> MFLIHFVHYKTILQKYTFKFKHIFLSIDKYNSLFFNISGILIWLNIIHINIILIKYSFFILINNFEYLIILIST;> MFRLTAASQKNLNSWYTKGTMRGGVPRIYYAWMRPGSFTRRRFEKMRNPFVDLETGTSLYFRDTRDSAEAIAHAADSKGIKGMDNAIDLYNEYRIVPDLYPEGFQWKHKLNTEYNQWRSNTWLTPDLIPKEHRGRFLCNFQLNIVAYDMRVVKFSPKDHRQWIYCVLYVGSGKGIAGWGRAVAPSTQEAKKEAIREAFSNIIAVDLEQEGPMYPVRVNADGVRVLLYPARRIVANFRVADILCAFGFQHAGCRINLKATNNPKSPTHTVEGVFEAVKALRSVSEIAASRGKVPHSLIYNIYPYLEEIRRRKGMMAMHPPGKDGLLMPDRVVDNRLPDHLKRGYYDDVYWKDFFAGSDEHLNEPRMGLRGDEMRRRLEEAQTSPAPTTAKDTRRRTLEDVLKRLGKTTRDLGSIPIVNPRVDVGLPTHIKRNYQLH;> MQKLLSPRTARHARLFRLAGKLADSGSPGVPKSDGERLVWVNSHVRRDKDISLSQEEERIRELMMPLEVGENSFAANGQATHGNLFYFREYPMYPGEYVPAEHNTLSSLRDELRLDLTAQSLKEAWMRVSGGVYFQSVDEYYASVDGLDAEQIGEVLAALFPELNCYEAQALVQRTLECISRPVSAASRQLSRTITAEAVGLDNAPGHYTNFLEWMGRLTETRAFKTEHALFEFSRRKFNRDDVRVMFENYRLMSKATLLADSADSYSHFYTVLKDFARKVAGEDSRHQIGVRIDEAEVDPETGIAVGRGCADGEKYHFTALLRENRDHNGIITVMGKPLSLVLDNKAWLMEMVLMPFDEANLDYRDFDAHIVSEGHAMPSIANEIAAFALRMAVANALVKLIPLTRIPLKKSGLLSVDRRRERGQFPGYLDGKKVKRRFAKR;> MVRRSHVVAYYWSRYRMPTQMPKFDGPAPVAAPQSMNSTKTNEFIDPIDDKFPMSIRGPLVRPDVPEDQYVDSWYICTSMTHHMGDYRPWSASAPPNAFRFRPFNEFDAKGREYVQYMREFARFDPRKSRGNGQKGFPFRDAYLTKMNEANQKTPPPTLETIMDRAVREHHQHARILSPLEVQRDVGRLEPIPSYAGKINADRSVFPFQWKTEDWYEYEVAKVRNRRFVFENTEEDGIRGSEVTYKIVLEGFWDHHVMKLAEDVCMFLKDVGRQIVEEKLVAVRRLLQGGAVDPELLAAFNCARAGPFGGLDEYDKEEVANFLRSDLRRLEEQCLSVINRCNVPVPGATNIYDPHTSWPHVEKLEPWVRMAEFWTSSSDTSFTELEMSTAHYEFRKFFRVIICKLPFQSTEFEKRMYDIRHWLHRQTSCEFHTIYRRNVIHDSAVFPTEHDPATPTTHEHHRMFSFALDWQSAPVNRLSTDTVHEGESWDAVAQRLGCSVGELKDANAERETIEAGVVINVPVTATRRLTSFGATPLVLPLKTTSAKDGERIRTWEEAAAILDCTVEELQQCNGHAALTYQKKESEAGEFDSSVTELVAPLSCWTSTSESEFSPVERVHANDTLVAIARRLQCSEEALRAVNDGITDVSGLDFVRVPPEARRPRRLVEPQLRPQAATDALLARTIAEEETFKLKSIPHLPQNAERFPHEYHTPTSRFPPTPSETPATQDWMAYTAKYLDKQFTISAEPAPVYNVNKLWPMQQIPGKVDQTPFEEDQTWLLHSIPVQQLEMHHHEKDLQDLPFINHEQFPRSLEWNAP;> MMRKSVTFLRRGKPRPRAGMFPDKYRRVPMLLKPQQGGQQYFNHFLIRSTNDRLTQQDVDNASGQAHSFISPQLPQMDWRNMSARSSEESIREEMRQLAENDVMQHQRVFNERMWYEKEEEHRMKARSCPEETSEHAISNDGAVPPPRVLGGDYFKTRFGYSLVKNSEMTQGPVDYSQLDMWGEMPRYTSDMVFLYLVSRRRNTYAVAYTYEGKRILNTYTAGNRGLKGGDRGFRSEGSTDNGHQVTSMYLNDLLPKLREMRASEGRPMGRGEKVELVVRVMGFYNGRQGAVRAVQDRANEFHVRYFEDITPFPLNGPKMPRGVFK;> MFCFSRGLWMRHIGQDVPKRHTHFVLESRLMYEKSFRDCWLHSVCRAISQLDEPLSKTVVGTHQKMLQRKVTCFQYNQYGLFKTPYYRLANVDRYHAVQGVAGTREWVPYVNVSYWTMNKMVRGGNLLVHRVHYTGWGTDSHLKKGGWEHRWNKVLQRNVLQYSRI;> MAFRNTFTTPGKFSTVSKNIVLLLIWRVKVFLRAEGFAHSLVMLPVSLYSKILLCDVKKKIVYFHCCTRKKSMLRRCPCVWPDGPTKSSVSIGTAFTLQKRFLKIAKSAFGFYLARRGQRKYPFLRRPHIKNTHSMNPSAPYFWSFMTAKSQMAFLPEENYITGDWTGKFFVSKRQVYTLQHATSGAKVRVKSFPSIFEFNSPSRWNIGKEMNTLTKPRMDLIDEQMLTKKQRLDYVRAGLLPK;> MRSKTLKKSLAAMYMRPPVTCYTDACEAPVAMWDGAIPLKETRKLKNGVPVRTVSRTYSHPPQLTPTQLSFNDINSMYCVGNDELIQFFPEGLGGRVFQTMPPGHPRGFLYRKETHLLNLFVDKVQHWHTKRSVLSSLTNGRTGFIVDGPTGCGKSALMCQVVHFARSRNIVTLYVPDAKVWTHGEWCWPSTILPGFFDAPDAARSFLKYFAVANRATLTSWKLRCTPKDLPTEQGERQPQNLYELCEWGHRAVAPASIDRQSVCVKFLMDELSEEKKLPVVIVVDGWNLFSHETHFRYPHPDFLRGLASFNESSTDIDLYPQELPRIPASRLSFVRGLNKMILSGDDPNKFFITCTTRDFKPFDGISGFPNVETDRFANSLDEYAPYDPEKDSHFHPIQIGNFDEYEYRSFLRFLINSGELAGLGWGPLWHASSDFERKLYKIGFLSGRNPQGVVDHYHQELVWRYDYQRTRQKQYLLKRRMEGMSRGASSGAVGVR;> MVLRRWFPLLGVHRVGYTHPSTLPVPCAQRWDLRLARARIFQEYIEEKAPGAWQLEDERSMSPEFKTFTGYPMRDMRPGYGQNLPDYIMKKRLPNNTHYELFARRDIPNEDNAMYGKYLYDMTVHGTSLPSTYRMHKDINKAQRNDRKLSGNRFKVLCSSGAKNPPSGWEPIPDATEEEED;> MRRWHRSLNPALFGERGSGHYFSTTRARLQLQAQDRIICGTHGAGIVAHQTAVNSSDNPMLSSVTTAAPAADLSRTKPHEGTGTSERDPYIRTLHNQRSAAPESSVSQSHTVNAPTVDECEMLAERWGTMNYWHNDTFPRLVVFLKKLLVPDVSPLSPTAESLLSMFEKVVIPKLTSDEEDRRKLVSLWSETTLQAEAAVTKFLFQRGSFESMLHRIITDALEKMSTLALGGQEGNLALEALKRQTLFKRNDYIQKRLIDVVSNSAYLGYGDSVWQVFFAAVEANEENLLSDRATTDAIRAAWEGVMREDVVRLPDVTGVVALYLTLVCIRESGRLVPEELKELSSGLEDGVRPGVRKLQQYPLIFLHPTVKRRFVVKAVAEILHNSSSNAFSNMLRENGLHDTAREVALCEAMNRNKELAEGDVGDAVGRFVSKGEVKTLLSSLVSGTDAVVRDAVAGIFGIGTTITIDWDAVMQNVDWSNNWQRLATALLSNSAVLSAIVKLVKNAIGAKGMSKHLFTDEYADQLQLILDAREERAASRKQRIENIAQELSSFERVDLSCDLLRKLGVDMTELDTAAAATRNMNVVQRPCIEDGLLSLVLEAVTKRHPNWVKAGVIQTTLKDPFDALRWMMHIFIRLSYVPHAGAATIARLSRRRIGPIGLEPHQFNVPAELGFVEQYDNLQYKRYDWQGWYQRMLDVHNRNVSLRCRICDLQRLDGNGVQFVDMQTERRLRILAQHRVGMGVLKLDADKYEDQADNVTFGTTKLSELLADARKAQLGEEYWPSVELKVRKPSGQSKAHYSLIDNERIEKRSRELYEKYRDAKKRSLFVTPMETWLEVKGMQVRKSVDNADEDGYTLDALQDMMDGDDGDKV;> MRAGCVACSRIPKLGIAALGSTTTSMQATCQETQELRCATTQMAPAVIFPLPPPLRGSYIDRKPTAASFNEHHATASFRHHMIASADVSHRPRHFYFASGTRNDTGTRSVKEGERKQLKQQTNVEVDSVAYGDQLDELSARWAAKFYGQVTFGPRNYPYPSSRWLARRFQMKKHRIIKRFRFRRYKLAAVANLPFAKMIRVGMLPELKSSKTKRGDVVDPTLSGQLVSAVKNTGEKRKGQRTRPKSKYQV;> MIRRRVCDGARLAPNIRATFSAVRYQSGLHTFIRDSKPSNFSSVRRSENANGDATASPGATAGENPASSGDWASHMQRELFGEVDPLGGQAHKDYYRDVTRGYSPQYAPRNFANGGAVAYPHIQSPYEYEEAAHRRVWLDHDVDRMREEFTQHRASLRSLASAQEREELLRSRAAEYQVANTVHESESVHPIQQLYNSGGTSRSALKQQAVADRYSIAEQHSPLPLTTGVDRDALDEAQRTKDRILNDSFTAENLLITHGLREKEKHDFTILQRTVRIPFQGYDMDRFLAQQKGTPYGAQQLPPNVVPSSMEEAQRTLRGSSATATPLVDAVAQKVYARNTVVDRPAIGEQLTEQIINIMRASRTTAEQQREEERAQRFGLGRQGALVQDGGPDQRTLKKHTNDERIVDAMLFQQNAYRKTPTDEHWNPYIRRSTENGVGHLLQNKFDIMRREDRLSKGEQDLTERNTIHYGVPIQQIVDEFVFRHRNARGERPLDYFKPFPNFRALRLNRMYRDVEGFSLMKQRPEFLEWELFTRYRQHHQQRRRLALLHGLEPVANETAQERDTRRHRLDEICERTPFDEREMRVNDDEMRVSVETLRSWFGVYMLPSPTVVNAVLGGSASVNLHLYHLADEMGTADTREHVLSSRYLNRLLLLESYQNRVGRGFMNHVVGRAPEPVVPHEQPQEVLRHFSAEERAMYEQHVKEQTSRQLGEWERAMKRRRWLTDHQQYGHVVSHGLETSVVDLSHTETGAVLTVSTKAYEQEIEAVRMKTNATIKVDGMVYNLLPNSERRVVPLTVQLDSGEKIDMTSEDFDRCELEAFPRNLNHALNYGIANYAYNRGNYVETQDSIWEEQTASGQEGWSPATHADGLREGLPVRARRPIFSSSAEQRIAGGPQRAVIIQYHHQPFFNPEPRLVKVAFQCDGTIMEVPISDVMIWQRRYHGPERTVGDESRRYNPAAMRRYVDVTDPFNEKTSNTEHFLDKYEPKRNADTVADKYRTTKQITEIDKWTRYDSARADNYRPLSISHRRDYIRMGYIPRYTPWEWIAIQEADQPLIAEQIRQDNIGTSYFFSLNRYWRYKASPHGYIRHFENEVRDLLQYVDGVTPWKQAQKIRTYWEVRSHHPMPQFNRPEVAMHRNTVGLLPAHMWETDKKTGKVKSVKDSVRDYQTKTPYPKWVQL;> MFRVRRLAGFIQCSPCGKMGPLKQQTRRYTPIWKSDPAVDNVAPLRDEDERRALWAEVGPISDVGSAVTAWIRFGNDPVLHTAVPTMLGGKFRNQQREKESLLPNSSSPFAYVEDYMGTNLVFGSPVHAKESAAVWATYFERRYASRLRLSRRTVANYVGLINSPEVFDDESDRPETRWSQDTFFRECAYLSEKFLKEKVSNMQQFEAALKRASPEAYLAFFDAFQQQTQTQIPLPSPSVWHYEGERRKQWAEKFISISHKAQAFFKDVLSEDVKKYQEVPGKLLQKVKPVLADVGKILVKRHERWLKGRVWTSLTEEEREAYCMKEVKRQQMQVEDGEFDPMMEDDVDDTELEEWQREHDAIMKLMNSPIDGLHFTTLELWLHTMRCEELETEHIYTSARVRAIQVAARKKLYDTTSYEEVIQAVVESIARGTLDLGAGVLRPHFNEVWCQLNYAKFGSSTITQHTTTSRRQLLFFHAGSLKDIAATATLYYATKPLSNSLDYASPYKYRRSLITLCSNYGVETAYTTQRPLLRSAANLARAEDLIHAVVTAAAQPFGERRRAATRDLHMEFQRLAVPVERVIVANPVSALLESGADPDEKPVEGEKVNMWPLGAKRVVLYKWSAPNVEKLKAMESDAASAVSGSSLTAKRLREIQELKRRGFLEVSLWRRVTAQERKQRNEIVEAKKKQVEEVVRTVPSLAHLHQYATSLYSRIEERVAFPTETSTVTETTNMKEETNKPLEDSEWEFAVLLDDRVLLNKEESVELYLPYRDANGELLAQGEYRALVRAFDLEANPNLHPAYCSVGYSESFQVFDALPQLIAQFFRVKDATAEAAGVTHIPAADFTPFCAFLRDAGLDVPLRCEFEAGQAVTTDGDVYMDYFLQLLRGEAFHQSHAQAGLTEAQRAIEPLCRAHWVVHHPGADESEWATARRSVLDHAMQHEREWWFPNEMLDVKDVVTGSTNGLTPQMYPAAVRYGVELCTVLTAEGKFVDERGSGLSARCVVNGTGAAESVVFDTANCNGTNTTSVEDALRVAHGALRSAQDRHNTLAAFRLGPLSKQSQVLLFCGVNAYEFGGKYARTYAYAFEKAKKELEATAASGFMAPSLSHEDTERLSDQPTTSPSVDRFASTTHPEQRKAQFVPRVGPGSTPLEDPAADQKSEWS;> MRRCSFASTCRYRSADDVPLGLGSAYVWTCRNITSRGQFNPIHNFSYAMERGVRARDVKAFEKLITNPGPLRVAYTPDYLDWLHRCYKAKGTYMDARAVAEKKFNGNIVSSELSAAVNRREGKRGDTRGDTVDNDHHNLPGAPPPGMFLRPAHSFRRLAGELKRRRAQSILDEVARAQGMLDLFERQPHFPAIHIDRCSRFHLVELFKEMVLERSLDSNMIWEKALLYRAILSERKPSYPTSFHYIFTAVEDTVFAPTISTPMEMAGSGGEGHDRSSHPLAAKCPTLEAYYYYVYLVKKYYIDNAVEAHVVLRCHREPNAADLLFSNPPPKDDTEIMKAVELLRNADIQRGVAAAAAVSDPTLPPGGEGSVIGNSDNKKNSEKTSEGSRGRPARPPVLPGAYPPIDMLWRCEENLPLLKVLLFGEFNLIVSENPFVKFPSAHGFLTRPYSTDSSRTLADGMSLANVMAEKRGHLLPSLPRNTATSIDARAQDIRRLQQKHHRDDIVSFQKLLRSTHAEDSPSAFSSYSDWSYFNPRAVRAEERDRLTRKAVEALKLYDSATNDIYRHSFEDVQACHTQRVTERDRTMPPYLPTLPHFVAIIKKDPHISFLLHIGLPDRNSSEEGSAKHKELEKRIYYLARALYHTALEYHNETVRRVNRQKVNVAASLLDNFVEQEWTTILRDKHDVTDVTKTLNDTQNDKKQLARRLGRYMLFANRSLDDTGFPTDARADDYTRWMAPPSVGKVSL;> MSVSGVFSKGRGIGHEATTSILRYIPRARVPWQPSRFGRENLTAADMARLWSRGRYRDGPGNYNSGYCTERTHVLEENTVSIIPRRELEKYMPDITIGPKALVTPVSLMNARNGHRVTHDLLHSYDPHIGRLGKPAVVDHDNITVEDPNRVGLNAATLDCRGRIYRWLRRGPFFQVDNYFRRSVKLNRDG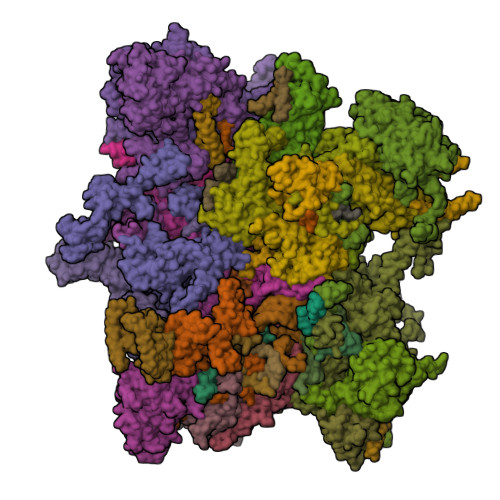TLPTDFVHEAPLMRKIIRLAHRGHLKAACEEYRRVTTVPPVEVYRALTACCVPGAKLADAVSIFEDGDSKLFYVSRDGEVLHNLMRCAIAARHRARIMWVYNVMRGRFYENVVVRAEVDLIWRYRIAMIALEYLLDHECAEEAAAIYSYLVEEELLRCDVHVRVGLHMREAIAAGKPITLNNDVMNATSLVRDATAVAPEVARELQRRHAQTLQNNAVEAVGAENVREGSAPWSILGPLTAIGPTAEDTMVWLQQHYGDVDVMSIMRWARFRKGKDLMAKDRPQYLARAAAWIELLSKRNREMEEVPLTYMRKSKPLVLDTNSNVRVAWQTPLMRSGGPPRLLAREEGYVFHHSNSSRFVEETYRHPGESLQSRYLALQPLHTEVSAKEDFQRLYYQAQKHHKQQERLLPVSTAAIPSRIVHHSVMSALHGVSGKGEPANRSLFTGNKSNDSHSNTGVASGTSACTDGAGSATPEF;> MFRRAIPLLSANIPRSVWDPAQHNPNWSDSYGHDITNRRAWPARKWTVGLEPCTPREWLQFSHRNLAYAYNGALRACHSLPSMLLLYKEMKQRGVKVDVDTMNVLLTRAARHEHIQVDDVFLLFDELVALGARPDLAAAETLHTVLSHSASMPEEWREARRLQLVELYNNLAMEEVERLAPHRADRLLKEQMKRFRGNLQQLGSGLRPTVYCRYLHTTHTAAVLLEEVHNFLWELVPNDHPAMEIPALQLRVPFVASVLRRPSVNPGVSLASVSRAEFGDTDVCAVFLAAAERMVDADFDDQRPVSERRLFLSLLTMISYSGVLYTSDLMAQLMEMVKYSNNDETRDSDAQRVLRYALRGSSAAQDSASRTLWHSVEKVADCRVVGRYIGARNPWNPIRVCFDEQGVFKAYPISTTTTTREVSPPEGNGAVTQEQRASCVEGRTLEALNMRWDDVRRLIECTGVLVTPPSERCPQQQKMEVFTGMAVYLRTVATGRRYEGGEDVLSDGAVATSSCEQRRRGTLFAEGYDFDVWVRLFSLVQEVRHDMEKFMADHTLQCVEPEFECWEALLVTLRCALDFCVVQMQGGGARGTEREVVERLFRDVVALREELIEESRTRFGGRMRVLWLQEA;> MLSQNVAKTTVPSYYMIRTNLPHRKPQNQWEGVYYYSGITKRQRHLILLHRKREREAHMRSFNISRASVLQRLEQLSGDRKQESLPPHVRLDLAVRLAQHGLYQQATPIVDELHHQKALHAGHYALLINALACPRLGQRILHCDAQCDPALTYKLLGDENGEERAQEAYRWFDLALTSLAVDCGGRTQPSHFVPYLPQGTAAASHITNALMRTLLTCGYTHVAAIPDSVYDRMGSMGISPTISTYELVMLALSLQGNMVEAESILSFLRSHHSEHITVESFNALLLGHREARQFDCCDAIWQELVDRRWPRASPLTAELYLRSIMDHANTPTSEPLQSFANINVVEKKKVPLVLAQMDELGVPRTHLSRVLMDEVEDSLRKFQTYRSRFYEWGRAVKQFDFIEFRRRNGWLYDLHLMKCTTKQVGPLRDFNDPDAVQGAVATAEIPAFFNERPAWERPPLEETLYVTTNKERYDDVRGGDIYYDDTRGLHDRSPTWMNEVPETRYDRLYGVNHPDIAKIGIRRHLNVEYVNRKEVVERDAALMKKTLSSGRRLRHRVESSRTHRNAGSLSGISSTAGGGSR;> MFRSTRPRSVGYTPVNPDTSPMVAYSQYHWHYNLPQGMERPHSVNRTFAAPFQSNHSLVNKYRGVWIEFDMHPAFSVALEPQLRKLPRGRTLPKTPAEEVIADYTALAPLVDDEKTRDLWLAKVFQHCAFQRCGGAMELWERYCHQRFTAEGATAKPPLSLVKSVLFYCNKTDNSGWRALFDRCLKDGWNYTPLFDTAQWSFMLKSIGRMGDEDGVRAVLEEMLDVQADLDRVEARSVVIALNAVTNADVYEFVKKYLFNFGERKVKFLRTTYSDLRGHGAGKLRIPLKENDNMYYHVCWHSSIRSPRQFSPRQLYFDYTPSTLGSSSHNPNAKIDDIVKDKIEKWKAEGLLPEDYVHEDRVYDRSAAFKNVARQEKWKKMPKILKSKRMGYTGDP;> MSFRYTNNLIGALKHRLLLESSYREIASRKFIGNCRGVEVVCSGYGTVLAVQLTDKAVWESFYRKGGRPTVSGGGDVSGDAETGTQGSATTTGATGSLDLDKLAESIKTALWDATRKIRSAKEAALHRSLSHNTRMRASADLKHWYEEDANTLRPLAFEALKHEAATPWMQLVQHGKKEEAAALLKEFEQKGDAAEATPTRVKDDRVKGTRTELSNREQPPLASTLKAEDSNPATIPIGSVHPLFTPALVQIEEAGGGSVSNEAVCRAQLWELSRDEQLFWERVELIRKGQVASIGSSHKRGYADEAAFAKDDTEEKVQLRFTQ;> MLVSYLRLQADRRTRHHMMVDGQINPREWFNWHPKEYQPWYFDRHKFLYEQRQYAQFHHLLCHQVYLKDMLHLMRYPEPYTHIIDCRTSTQKMHRWVPHSLWLPRDEVEYALQLSADEFLDMYGFRKPDKSDDVILLSHNGIYSEQAGWEWKKQFFQHVYNYRGGTNELFGESYSDMNVSDVLSPWKGPFPQSGVFVDKWSKRKVLTRTGPFDRQYEMQDFALPDLELEKARHPEEGPRQNMPFGLQ;> MRRVRDGLFLSHPSSALQCSVAVVSTGEFDHPPFQFRQRHTFNTTPLHDANRFGGRTAYLREIGPVNIKKQGRRFKKDPRTVQFNVDVWCAQQTLRKRWKQRDWEVIEIPFRLVPREQQRVIPELYTDIPQMTDPARNDFSNIRNKVYDREELQGVLFPAAGAMLYPPLQRVDKQAMTLDKYL;> MLRFTHRALTATPERFSVLGTTHPKPKRTGFGRNNKMRSKPSDNVAWYDKGPVEWLPRPVRLTYDHLDQLQQWTMRATLDGRTEEFNRIRDLHREWSQHPLMPVLGDVEPKFPLNLFKQNHRAKKRFLVRWHKANTPANWLWMPRGPTVVTPLHRTNPTQYPENWKQMVQRKSGTGTPS;> MFHRAFVSSSDLTGCTIALSSVCTQKRYWAKPKKRPKVGQGFHEKAQKWREEYLLDRHRALADSLRAYVEFSTSKRVEPWDARFKPFDRIEKDGVYVLMRYMMEEKLQLCNYHHRPVKRLFCNIGLMGPQITTKARWKPYRFATNPAGTSKAERMYQRDKTVYTHGHND;> MLRSTLTSLNTFLTSSVATPPISVIRTGPKWWAHPERMVRQKLMYFTLGVDQLPLRRTAVIQRDLQRFHMCKPPPRVGDSTGYKRSRAAQLNTWYRRIQYQEYHMQHLFTRHVWGLLRVYPGNTTKIQGKADDGYVGYDSVPFHRYNRAPLPFPARELYERRK;> MFFRFHSTTLQTCLTSGVARSSVAVAVPLRAGCTRREMSSGGDGVLEGAMHKPGESGLQAGSSTTIAGKETWSQFSTKMRYGRRRIRVIDVAAKMSYEYQMLRKMCKRRPAMRQWAVRDDFCDMNPGVVIMSPSMQAAFMKVFRMKEKGLIRQCLRDIVPVIEYRNREEPARLPTNPADMIPEGEPDTLNQKKRELFERREKGENFADLRLHDKRSQAKLRFRIRQRLLKFQRQLAVANAIASRSVLYSTNDAIGYFLFRGAAMYAGMHRVFFELSKQLPHFVPKTMLDFGAGTGTAILVAKEVYDPGSLAYPLYRSLRQTMQGNDSSRTHQLSELRYDLKRLQRNNEEKKKVRFMAVAALLERGEVDPADLPEDLKREIAEVATAAATAKKDRLVREAHARYRDVVDGTEWESGDPLGEVRASTEDPEDVIDGEQGDGGDDGEAAKGRPKTWWEKLIDVENETARTRAARRLRPLQEVTAVEPSPGMMEIGTMVLHDDVPNVTWKRYLLPEDEAIQHDLVVAAYSLSEIATSENRRRIVQQLWKMTKGVLVFVEFANLNNFNILMEARDWILEEKDVGLWDWQPTIVAPCPHEHRCPLRHCKTGVKRKRMRICSTEAHYRSTFVEVWARHMPLKVGIEPISYLILARNELVPERAERRREQLKKAEEMKRRERDVKQQQLHEASLAVKDVVFERLSDEALHRVQSSVPQPLTDIDEVREASTSATSTSLLKDLKDGATSTGEIGHMPTDVPRLVKTGNTRHNRLIFPLQFPPATHKFNRAFVDAGYQRQRAITPAEMLVVRQEVEQLQQRVMRAAPKYLRVVRDPRCHGKVQADFCTPEGDLVSGRVYRRFYGDRNRVSAHSTMRWQHIGGWKLLKRIRRGSLFPHNVPLYAVTKHAQIDFPNTLLDTKHSTVEQTAMQYNDPMSLVEMPDDGLTREELKQKRRLQRDVELQKKVEEKLEDIFGVNAKDWKTDDLGGGRLDARREISEQQWADAVRRAKIRTVQHTKNALPFAAKKRAAQRALQVRRRNVRLEMSGNRRR;> MRIATSPTRRGKNSSVLPLLRRFSWGNGMCSPYYTEHRRQSTLTSSALSSPANHNQQVVYRSIRDCRERAFHLIQELVSSPIPGCGLSYSTNGSFGGPSLTANAVSGVASLLELYDKAYYFLHLLHRTILVPRNVVRDTDDFTEFLLRCFRRPSDSLLKGDEELQLSDAAIVDGFVEWMETSLMSAGQFVSFVEVLQLVGSYVRYHKGVRWGARPSEEEWYRCGYRLHPWHDTYCPSSRAEQMPYVHLLQWLMRAKPTKLEEKIDNKEGAHGASSLFSTAAKESAMRAWYATEEFSPPSWHTVVGNSNRLGFTALDCGCHSGYMTELLLKAGAQEVLGVDVSPHHLGNAEATLSEHLRERRSSSHSRKTVQFVRCDILPDLSDEARQTKTPPLGPEGSTNSAAAENRRRLARCHHMPSDSDGLKTETEVTGPFDLLLFHPPLPLLFPTWPLFHDLYESVDQLAYDAGRRHPHCRLSVLNEFLQRLLGSSNGEENNSERRRNAHQQLKHQRRLVAPLIKDNGYVAFILPRNFDTRAILQRMSTSSAGKNCTSCGSDGLAPLVPLSDVVTMTLEGSYTLVLKRSHSLSSLLNRMDYIQKSISAFIRAFVSPQHRSRVEQEVRDFYSNHQAIDLIVMRKIARQKTNEDNNNKDCSVRAVLQKVSEPIAYEDSFEYEEYIPAGGSPLAHHWTEMTPSFSYLEDEFFGCADSVGTNGPPNGASFLAVGHPLVPVTRQLVGVDRFGAGGRDATQGESGNFDKMFAKEMRRRGGRMRKMALTPLEKQEWYIDEKLVKSEAAKVDLMNELSRFELKDFD;> MLIRRLRRPHSTVRGCRISSASNSDSAGAFSANGTQLPDPPYYLPHSPRFDAERCGTFNKKWLLNLPALKPLVRNSTYLPKKEELWRAPTHEALETIIGHLPYHDALRYITEHSLFLLFPTVLRARDAPLPHVIYEDFMKSCTFASLQNPPEEQFALPSVLLRTLLCMAAYHCTLDADYFTTCQMLFGRMEQQQQTTPEVLSAWVYCCTASGRVDEALTYAKYMADCSAPFDVTVFSLMQHPSLNPIEVEDGSVPHSAKGLLLQRRLGNRLHTAYRSDAVAAHGMFVYYALTLSHVRKWEVIRAAAALGVTLAERTVVLAVEVFAREKGMRCGPKTVKALTHFLAQDGTVGHLLYVLLRARKNELLPEFRDLPHTTFSEEEQELVLQCVAQRARHDDSFAVAATLVSSLVREDDPSELLMAFARAARNHHSADVCGGDGDGSVCADVPAPVPESPPSNSSEIIEKDRWAVVQASVRSLLLDVNALDQASRRDAYHKHWKNGNKGVKNKENVLAKTLTLPHDSMHTATIQRKEKELWELMRSDTPVGVRELAQLNIMEELQEAKRLERAEMAWVNPDGTF;> MKRIVVPHRWSEMNRVEHPPLMMKQLFQGVCGGLRWLETKSLAQYLAVRAIEEGYPSTPGVRKALHVKRAPLQKRRVVQRSTKSATAACSLPTTAAPAQLPLTSSGDALTVTGGLSLQVTKQKRLVSYDVLDCTLGSGYHAGAVLENGGPYTRVVALDCDHDAMHAARDLVEEFGGDRFRFYCCKMSEAKAMFGERSFDAIMIDGGVSDTQLEDPERGFLLDDEGGHRLDMRFGPQMGVGALEYLNTVSQHTLVSSLLAYGLLEYGQAMKMSRAITRRKPFVDSREVLTCIEQAGDELPEGGWRSQGSRRKSPMSWKFLTSLRCIINNEMYELRQGIENALLMLRDDGRLVVFSRLPWEERLVRGTVDDHPHALLSYVEDISIDDVQIYGFTRHAKMWVITRAASSAYALKNTTTLTEEKFRESSVRWLTGMYAGQTHGFPANNFTFENFERKEWVTLRRNGKPPPVDVGLDDK;> MRWSAVLCKVSKVPTRSVIPADALRYHPRYSVPRKMVLSNTFNVVGENNRYTSLKLILEKLSGHVGRRQYKMLCNLEKHYDKLKDEGIDWHELKWLSREELIVLFDKVLHLTRTERAALLPAIEAKVCGVLRQTDSRHSTVVCMNRGNANHGWRCGRNGHTNDVYFEGKAKANTAALQLCRRSSVRSVERSGVLVEVRSEPDFSVVGRFDHSLSPRVWSTPENPTFQVTTIGYEFRVHQEDPRVIPQIVEAAEEWELHANITKQVIWEMLEMYAVERDRQPLDLKPGEMGDPDIPSRHATAFNVQVVPPLSEGDEAIQVVEQRIVRADGSEVPWFQEPPPQLFSGGIPVILPFAPSIIVKSTFRQVTRSSAQDVTRQLLQPVVDVTCFLHPNVCFWWNAEDEQRCLGHIVDYAKRIPFALPFNLYFRVNLSKDLRGVQNYTEELGKRMSMKAHYFNLRSYGVR;> MLVCCRSSLSLLARATMPLCCSRRFLTHQNNIDDISGPVDTNSNSVSDGRLHCSTGEGGKASTCERVSLRTIAESLGAAAAAELRAEVERDTRDGVAAIPPLPPLGWRVRHPSGSNYFVMTRTLKNGVQSAELNNRRYRSVHDIFLQSLQKGGHKYAQKGKGSEGRQKDAKEEEEPPSQEDGKSSPKVTVGYDREGRGHRATLQRMDELHDSPKLSRADVHLTVFAPFRVYDPSLHDPTVDICEWSSFDLVVQKTVPDNMVANKLLQPLSCTPQDGALSMYVCLASVNSEMRIRSIQLLSMKEAQALVEHACFGNGEPLFLELLRRRGRRRPLVERRFDDPRLRYEEVAQPQQVADEAAVACSSSCYGPYYPAFEMLMDSCGSAGEYSRALCYGGPYVSELSRELCDALLDYIKGDLGVSDQLCEYVCQMQFFLEQEEYMTWLGQVQHVANAVSRTA;> MQRTLRSAARRKWGQKTWSPTATNGGAAPANGVSAQEALQIAYRPMPPSQTVEYEEDFGHNLMIHREYISKRCRDRVSFELSALSYSNLELRRGQEHLAGIMNRERRGVSVGASGAPDDQVQMQTDVDANSREVLSARYLFNERRLQFCDRFQNFFQSKLENSAASDSNGHEKQHLFSLMEACAVIFGCETEAARETYYRMFLGLDSETLLEEDEALRNRIADAKLVQRVLENNKGRQEVTQSPKLQQQQDQGKPLHAVSSGTSLLNDCEEERFISSIPELSLFEDETEARANGFVEGEDDVKANNGDLTAGSFSSPASSVNLPEEFEEYAPLYKAYITHAVGKGPVASYDISTLGSTGLTAERRRWRTLMEKIVREDYHTMTEVEQMDAIVLNEQLHTVKFFDLKIGDAIRDILQLLQRETGVGSSVNRDTPVGISPNNPERRV;> MLCHNRLLLVNKQTQKYRTKLRYRFRQPSVVPLRQTLQQRHNTILEVLRRRRINSGDQSPYRYVEERLYSKPSRLDREGVKVNKTYALQGLGDLEPLRYGANFGISEKDALKYETVAEKAKYMEPPIPYSSLAARKLAAGALWPAAPDPEGMISKEVRLLRHESSMSPSARAFSERVAYHLRRSLKACPGHIAEHIDFTQLIIQEVLGSRRSKEIYIVWFTVDPGARFELEPRLHQLNHWVQQLIIKRVKRRPHIPRVTWIYDGGRLERELPRDVKQELQSFVADAATTLESRVKYLKELDTMNQRMKDIPWFMPYLWSKEEKAARQKSMLADLEEVERRKNEHSSGRSAPPRTSPPPQFVR;> MHSSLIILRHAYFSALHPARRVVPGSLLPVRTQFYTRHFTSTAGPTCGDGGETYKSEPTKVGASVEGTNSGNGVTDSPSLFSSSAPTVRRRALPPSDFPENALLKCIEKEIEDEALRLDKEECPPPPPTGWEMYHAPGTSVFYGRRWWLPATASAETRATPERHTIRVQLTKRDPSLDPECDVRGEHFPFSFFVQRAPSKGEAVRRDGTFRMGDSAAAGDVKGRTEGKEEEEEEEELGLYDQSIEVRADFVDGELLVDNVVFHGTFKTGSSCSKRSGNTSPEAAAATAAGQHDNTTGGRGKVEEVRYNNIFNGYPGPNLDEAEEEVLDGLQAWLAERCVDDQFGEFVGQYSVWVEQQEYEMWLKRLRDFVAA;> MRHFRLNRCSYTPNLTSLTNQVNRSERLRKWGSAGVPPGVPRIPRLEAKGIAILHESPKVILAGRSRCNNFDSNQYMLINKATKRCLLVDASDDWPDDWAAFIGASDLTLTHVFLTHCHIDNIINLNAFLTICGSRQKQRVQVDSQDNDNREDDNGSDEIGVMWCPAEECWVQNFKRSCERYGRFEEMHQVLPMMCRSLYTPQHLVDPVIAGFSRRNARHLRRNDVLLSAATNRATSFIDFGNGVLLYYIFSPGHSPGHMMLHIPTERILFSGDLLFFNKVGRVDLPWATGVRLAESLRLLEALPDNTVVVPGHGRMTTLGRERRENKALQQCYQRQEIGKQEVSVGFNEGYL;> MMKRTILQRCIQNKSLEIARISRSDINSRAHLPFNFDVCYELGSREFTLFSSVGSTSVLVFCNVSSRRLRSVKGGQGETEFPPKRLNVKRRRQSGSADRSPVVFSAFVSMPTSGLTIEALCCSSLGLLVVDGVSFHQGPLTESMIPQDAHPGPEGHYQGPLLNQRSLAEMVVNTRGCITSVDPFRQQESFFDGHVNPWNARSLRFGHVPVHTAKPGFSDALCHFLEVFGVNDELAFFVEDFAHLVHREEETAWTNVLKTMMGGR;> MWRLSRSLRSNSLHNPGPFLDGALQLIKLHLAHKNAAADKNTKACSDIEGEFLRELEAFRACFTMSSSLKVAKLYTKKLHGALSYFQLYDDPLMRQLDMIIGKQTMQPSAGRQHGVFKAPVAARLDPFFLDEREETVLPSELPNPPKPDPSTPLRERALKVPAQHRGHWVLRDPDIAITREERRTDPW;> MPPNSATRWLPFVSSDLKDYLNRYWAVMFTVGARPIETGHIRHYVSWYCTRMKVVLLDHHVYVEPLRQQLQEASRTPELPLLFVNKKLVGTLRDVELLEREKKLKDVLHFGFEWRVGGSVAATNGQKSLMGALPAPYGDAEFFRGRYRGPPVARPVVSLPTLHPFALRSEE;> MSRSTVFGPGSLYSFTKFGSFNRSPTNCTLNKRMKDIFRLENQKHIRNDFDRERRYRMCTKCGITTVTINFNNVPSARVGLWGRCADDKDYTHHRMVDITQREYEVLRESPVEKRLNWWRYER>[2x]ETPVLEKNNVTLTGGGENVTKELKDKFTSGDFTVVIKYNQSSEKGLQALFGISNSKPGQQNSYVDVFLRDNGELGMEARDTSSNKNNLVSRPASVWGKYKQEAVTNTVAVVADSVKKTYSLYANGTKVVEKKVDNFLNIKDIKGIDYYMLGGVKRAGKTAFGFNGTLENIKFFNSALDEETVKKMTTNAVTGHLIYTA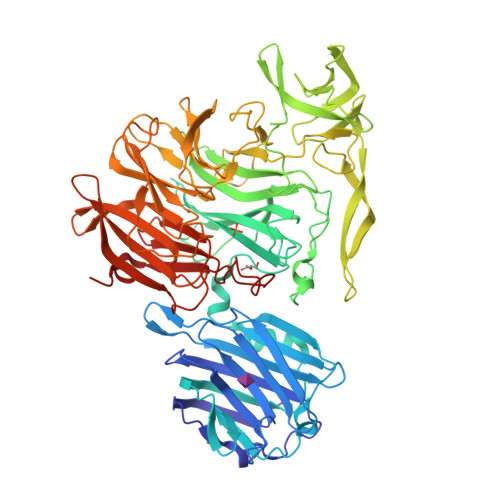NDTTGSNYFRIPVLYTFSNGRVFSSIDARYGGTHDFLNKINIATSYSDDNGKTWTKPKLTLAFDDFAPVPLEWPREVGGRDLQISGGATYIDSVIVEKKNKQVLMFADVMPAGVSFREATRKDSGYKQIDGNYYLKLRKQGDTDYNYTIRENGTVYDDRTNRPTEFSVDKNFGIKQNGNYLTVEQYSVSFENNKKTEYRNGTKVHMNIFYKDALFKVVPTNYIAYISSNDHGESWSAPTLLPPIMGLNRNAPYLGPGRGIIESSTGRILIPSYTGKESAFIYSDDNGASWKVKVVPLPSSWSAEAQFVELSPGVIQAYMRTNNGKIAYLTSKDAGTTWSAPEYLKFVSNPSYGTQLSIINYSQLIDGKKAVILSTPNSTNGRKHGQIWIGLINDDNTIDWRYHHDVDYSNYGYSYSTLTELPNHEIGLMFEKFDSWSRNELHMKNVVPYITFKIEDLKKNL> MGSSHHHHHHSSGLVPRGAMNEKLAKKKIVSIDAGRKYFSPEQLKEIIDKAKHYGYTDLHLLVGNDGLRFMLDDMSITANGKTYASDDVKRAIEKGTNDYYNDPNGNHLTESQMTDLINYAKDKGIGLIPTVNSPGHMDAILNAMKELGIQNPNFSYFGKKSARTVDLDNEQAVAFTKALIDKYAAYFAKKTEIFNIGLDEYANDA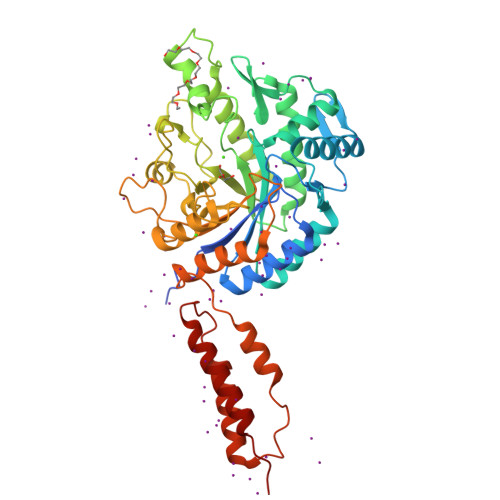TDAKGWSVLQADKYYPNEGYPVKGYEKFIAYANDLARIVKSHGLKPMAFNDGIYYNSDTSFGSFDKDIIVSMWTGGWGGYDVASSKLLAEKGHQILNTNDAWYYVLGRNADGQGWYNLDQGLNGIKNTPITSVPKTEGADIPIIGGMVAAWADTPSARYSPSRLFKLMRHFANANAEYFAADYESAEQALNEVPKDLNRYTAESVTAVKEAEKAIRSLDSNLSRAQQDTIDQAIAKLQETVNNLTLTP>MTPNWSELVAAADPALVLPSGERRAEVAVPGPLRLDALLDLGEGHAVGVVRSADAARWTVPLVRDGAGGVRRSRPGDGTAEHLVAALARRGATPDAAFVLEAFTGAAPVTGERGIIVDQTNESVIVGECAVVKWAVRLPAEGEPGSPAAQRIAALARGGFTEMPRPWGLLTLAEGAQPVLLASVVAYLPGALDGWDWAVDDVRRLARGELTMDQALLPAAQLGTLTARMHAALAARGRTPATAADVAAWGVRMREELDEAVASVPGAEGERLKAWAPRIADVYAELDALAGTPLIDVH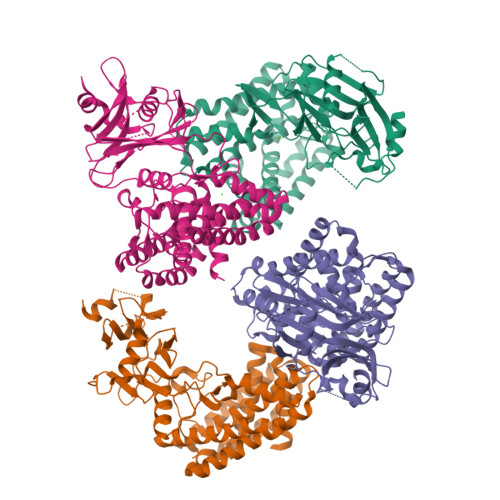GDFHVGQILRADGRYAVVDFDGNPVLPADQRAARQPAALDVVGMTASLDHVGRVVVFRTPDVDPAPVRAWIAAAQRSFLDAYRTTLARLDADDLFDDRLLTPLRYAQEVREYLYAVRHLPHWVYVPDLSLTDLLPERLKDKLAAALEHHHHHH[4x]> MILQLFRRKSKANEAIVLRVYEVIVAAARQKRFYAQFQVPDTPLGRYEMLSLHIFLALHRMKGENPALNALAQEIADEFFKDVDHSLRELGIGDQG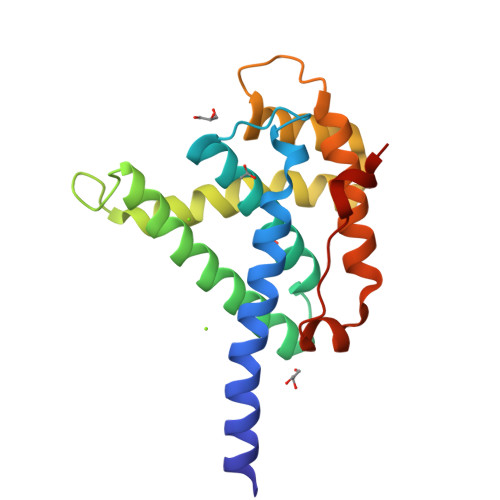VPKRMKKLARMFYGRVGAYGAALDANDAQALAAALTRNIRPDLEFWPHACYLGAYVLQCRDCLREISDEALAAGDISYMDVDQVDLAP The S. pombe orthologue of the human PAXT connection, Mtl1-Red1 Core (MTREC), is an eleven-subunit complex that targets cryptic unstable transcripts (CUTs) to the nuclear RNA exosome for degradation. It encompasses the canonical poly(A) polymerase Pla1, responsible for polyadenylation of nascent RNA transcripts as part of the cleavage and polyadenylation factor (CPF/CPSF). We report crystal structures of Pla1 in its apo form and in complex with Red1. Taken together, our data reveal the molecular details of recruitment of Pla1 by Red1 which leads to hyperadenylation of CUTs, serving as a signal for exosome-mediated target degradation.

To first gain insights into the inter-domain arrangement and interactions between the NTD, MD and RRM domains of Pla1, we determined the crystal structure of the protein in its apo form. The crystal structure of the full-length protein shows a tripartite domain architecture of Pla1. Briefly, the N-terminal catalytic domain is homologous to the catalytic domain of other nucleotidyl-transferases forming a five stranded mixed β-sheet along with four α-helices. The middle domain is formed by a four-helix bundle which is capped by the N-terminus of Pla1. The C-terminal RRM domain contains additional secondary structure elements extending the canonical βαββαβ topology of RRMs44. It comprises additional helices α14, α15 and β-strands β8, β9 in the extended loop L1 connecting the canonical RRM strands β7 and β10 compared to its homologues. In our crystal structure, 18 residues of loop L1, loop L2 connecting β10 and α16 and 25 residues at the C-terminus are disordered. A large interface is formed by a network of interactions between the three domains of the protein burying a total surface area of ~2982 Å2. The tripartite domain architecture of Pla1 is held together by hydrogen bonds between the interface residues of the domains.

> MKHHHHHHPMTTKQWGITPPISTAPATEQENALNTALINELKNQNLFESPAESEKRVKVLDELQQITTEFVKKVSLAKHMNEKMANEAGGKIFTYGSYRLGVYGPGSDIDTLVVVPKHVSRDNFFQDLEPMLREREEVTDLAAVPDAYVPIIKFKFLGISIDLIFARLSVPRVPRDLELSDNNLLKGVEERCVLSLNGTRVTDQILQLVPNRAVFKHALRAIKFWAQRRAIYANVVGFPGGVAWAMMVARICQLYPNAVSSVIVAKFFRILHQWNWPQPILLKPIEDGPLQVRIWNPKLYPSDKAHRMPIITPAYPSMCATHNITLSTQTIILREMVRAGEIADQIMVKALPWSALFQKHDFFHRYKHYLTITAAAKTAEAQLKWAGLVESKLRHLVTRLELVDAIALAHPFNKGFDKVYNCSSEEEAQQVASGVTLEVAYESTDHEKLANDTVNEEKADNTESKADGSENGEKQIFPVYTTTCYIGLELEKKKGHPIKRLDISWPTQEFYELCKKWDKYDDTLMNVFIKNTKNTALPDEVFEPGEERPKATKKRSTADTAHSTEQLKRQKVSTA>MALSLCVLFTLASVVSGHVAHPSLGRGDGFPFLWDNAASTLDQLNGTDTTIILNGFNYLDRLSMFKTVLEGTRKYFDSFAPNNTANIYWGFTIYLNWILATGRSADPTGHTTCGLAHGDPMCLAEESWWNCIKYNPAAIAFFAAKKAGIFGDVTKTIVLAKPKEANSPYCSSEEECQAAYPDVMATYLDYFEYL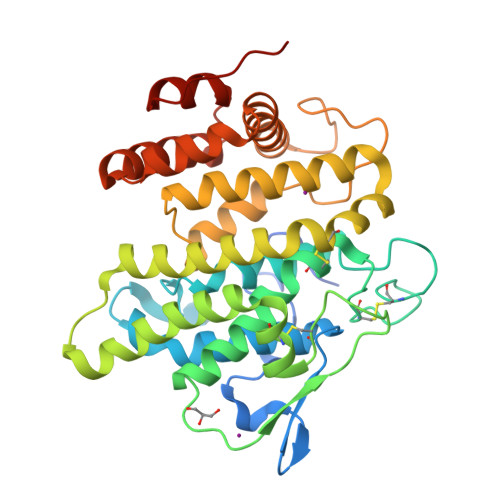MSLEKTGESIDMDKAQQLLWKAHVTSMENSIAVCKPRLKNYNIIERQLDRDYLISLLYFAATNFPTNFIESIKFVADMPHRQLRFGDIAPFIPDMDMKKNNLLVVLHGFYTVHSLSGGSSLTHWRNLMESPVSREMARDMVNLILAGTPVEVQVELAKLGIPTPVDYKDDDK[2x]> MSSFKYKNSAAGASMQSAANITLRQILEPNNVNLRSKKTHIVCTLGPAAKSVETLVKLIDAGMDICRFNFSHGSHEDHKEMFNNVLKAQELRPNCLLGMLLDTKGPEIRTGFLKNKEVHLKEGSKLKLVTDYEFLGDETCIACSYKKLPQSVKPGNIILIADGSVSCKVLETHEDHVITEVLNSAVIGERKNMNLPNVKVDLPIISEKDKNDILNFAIPMGCNFIAASFIQSADDVRLIRNLLGPRGRHIKIIPKIENIEGIIHFDKILAESDGIMIARGDLGMEISPEKVFLAQKLMISKCNLQGKPIITATQMLESMTKNPRPTRAEVTDVANAVLDGTDCVMLSGETAGGKFPVEAVTIMSKICLEAEACIDYKLLYQSLVNAIETPISVQEAVARSAVETAESIQASLIIALTETGYTARLI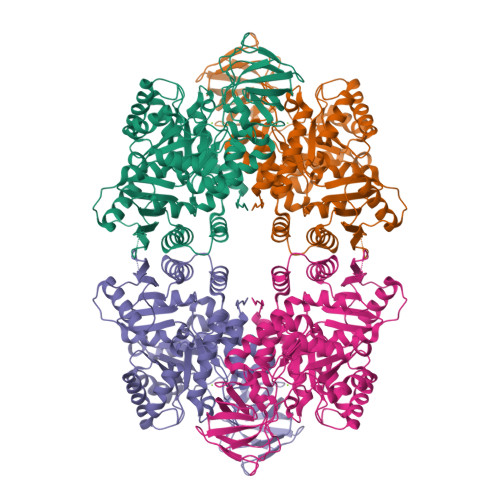AKYKPSCTILALSASDSTVKCLNVHRGVTCIKVGSFQGTDIVIRNAIEIAKQRNMAKVGDSVIAIHGIKEEVSGGTNLMKVVQIELEHHHHHH>[2x]PYTIELIQPEDGEAVIAMLKTFFFKDEPLNTFLDLGECKELEKYSLKPLPDNCSYKAVNKKGEIIGVFLNGLMRRPSPDDVPEKAADSCEHPKFKKILSLMDHVEEQFNIFDVYPDEE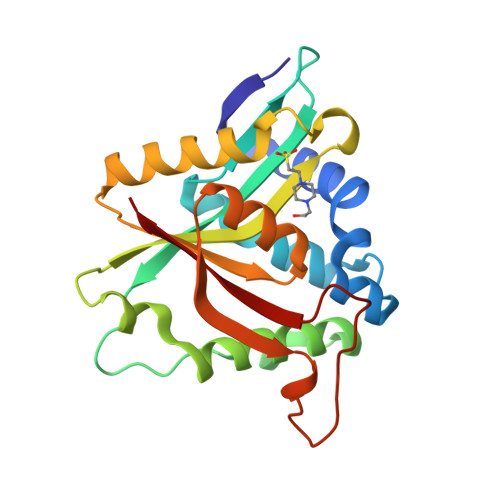LILDGKILSVDTNYRGLGIAGRLTERAYEYMRENGINVYHVLCSSHYSARVMEKLGFHEVFRMQFADYKPQGEVVFKPAAPHVGIQVMAKEV>[4x]GPLGSMATTADSAVLFYIVASQKKLSFDYTPNWGRGSPNSYIDALTFPRVLTNKPYKYRVVKAGQDLGVRDSYSVQSDGSQK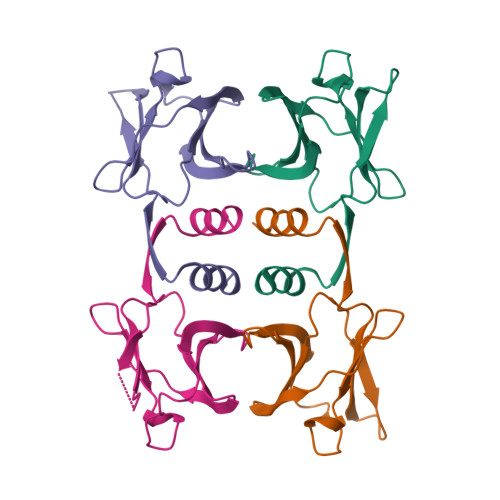VNFLEYNAGRGIADTQTIQVYVVDPDNGNQYLVAQWKHHHHHH>MRVFHFSKLPLGVAILAASSSVFAVTLDGGAVAAPDQYGAKVAAEILKKGGNAVDAAVATAFTLAVTYPEAGNIGGGGFMTLYVDGKPYFLDYREIAPKAATKTMYLNEKGEVIENLSLVGAKAAGVPGTVMGLWEAHQRFGKLKWSELLTPAIGYAQTGFKVADQQYQYRQDAIALFNGKTNFGDYFGTMKPGEVFKQPELAKTL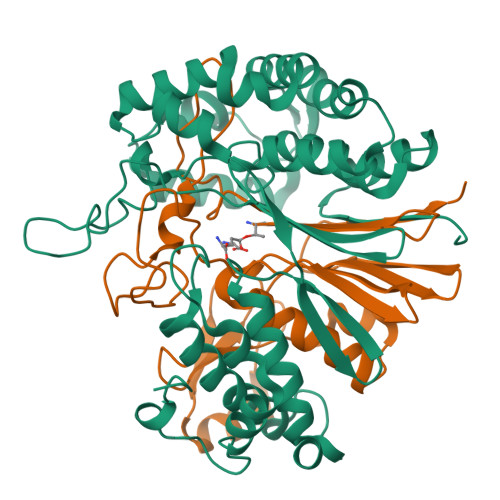ERIADKGPDDFYKGETAKLLIAQMKQDGGLITSDDLVDYQAKWREPMRIDWQGNTLYTAPLPSSGGIALAQLIGIKEQRAADFKGVELNSAKYIHLLSEIEKRVFADRADYLGDPQFSKVPVAQLTDPKYIAKRAGEVNPDAISATEKVRPGLEPHQTTHFSIVD[2x];>TTHFSIVDKDGNAVSNTYTLNWDFGSGVVVKGAGFLLNDEMDDFSSKPGVANAFGVVGSDANAIEPGKRMLSSMSPSIVTRDGHVSLVLGTPGGSRIFTSIFQVLNNVYDFHLPLEKAVAAQRVHHQLLPKDTIYYDAYAPLTGKVADELKAMGYTLEDQGWNMGDIQAIRVNGKALETASDPRGRGVGMVVKP[2x]> MNRNPDQNTLPNITLKIIETYLGRVPSVNEYHMLKSQARNIQKITVFNKDIFVSLVKKNKKRFFSDVNTSASEIKDRILSYFSKQTQTYNIGKLFTIIELQSVLVTTYTDILGVLTIKAPNVISSKISYNVTSMEELARDMLNSMNVAVIDKAKVMGRHNVSSLVKNVNKLMEEYLRRHNKSCICYGSYSLYLINPNIRYGDIDILQTNSRTFLIDLAFLIKFITGNNIILSKIPYLRNYMVIKDENDNHIIDSFNIRQDTMNVVPKIFIDNIYIVDPTFQLLNMIKMFSQIDRLEDLSKDPEKFNARMATMLEYVRYTHGIVFDGKRNNMPMKCIIDENNRIVTVTTKDYFSFKKCLVYLDENVLSSDILDLNADTSCDFESVTNSVYLIHDNIMYTYFSNT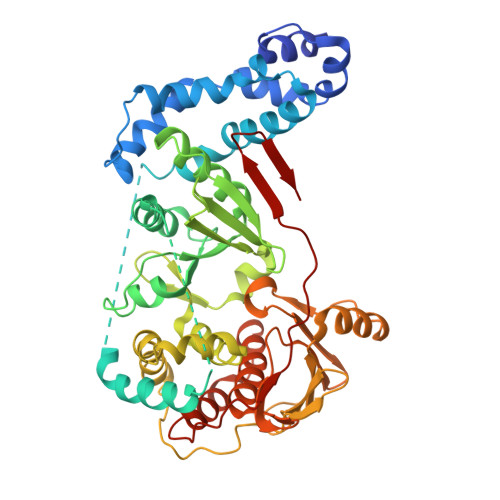ILLSDKGKVHEISARGLCAHILLYQMLTSGEYKQCLSDLLNSMMNRDKIPIYSHTERDKKPGRHGFINIEKDIIVF> LAPNDPYYQEYQWHLHNATGGINAPSAWDVSQGEGVVVAVLDTGILPQHPDLVGNLLEGYDFISDASTSRRATNDRVPGAQDYGDWVENDNECYTGSVAEDSSWHGTHVAGTVAEQTNNGVGMAGVAHKAKVLPVRVLGKCGGYLSDIADAITWASGGTVAGVPANANPAEVINMSLGGSGSCDGTYQDAINGAISRGTTVVVAAGNETDNASKYRPASCDGVVTVGATRITGGITYYSNYGSRVDLSGPGGGGSVDGNPGGYVWQSGSDAATTPESGSYSYMGMGGTSMASPHVAAVAALVQSALIASGKDPLAPAAMRTLLKETARPFPVSIPTATPIGTGIVDAKAALAEALE

Through the COVID-19 pandemic it gained more prominence by being a key pathogen in respiratory co-infections. This study will present a structural analysis of StmPr1, S. maltophilia’s main virulence factor, an excreted serine protease. StmPr1 is a member of the subtilases family defined by Siezen & Leunissen et al.. It shows the main structural and functional elements of the family, such as a reactive triad consisting of Asp42, His105, and Ser28922. The catalytic triad consisting of Asp42, His105, and Ser289 is located on top of β1 (Asp42), α4 (His105), and α10 (Ser289).

Bortezomib is a proteasome inhibitor, using a boronic acid residue to reversibly bind at the active serine of serine proteases. Accommodating the low solubility of ammonium sulfate in dimethyl sulfoxide, the solvent for Bortezomib, we adjusted the crystallization condition. Instead of 1.8 M ammonium sulfate, 0.1 M Tris, and a pH of 8, we used 0.9 M ammonium sulfate, 0.4 M lithium sulfate, and 0.1 M sodium citrate at pH 6. Despite the changed conditions the resulting crystals show the same cell constants and diffracted to a similar resolution. Additionally, Bortezomib is stabilized at its position by Ser176 forming a H-bond to the nitrogen of the phenylalanine part of Bortezomib. The oxygen of the peptide bond between pyrazinoic acid and phenylalanine connects via H-bond to Gly178. Moreover, three water molecules stabilize Bortezomib through H-bonds with the nitrogen of the pyrazinoic acid and oxygen of the peptide bond connecting phenylalanine and borono-leucine. For Bortezomib the P1 site is occupied by the methyl group of borono-leucine. The phenylalanine is located in the P2 site, while the pyrazinoic acid occupies P3. Therefore, Bortezomib is a solid inhibitor for StmPr1 using the combination of the pseudo-peptide structure with the strong binding capacity of boronic acid to block the catalytic triad by binding the active serine covalently, while the bond is supported by His105.>RFYVKDHRNKAMINLHIQKDNP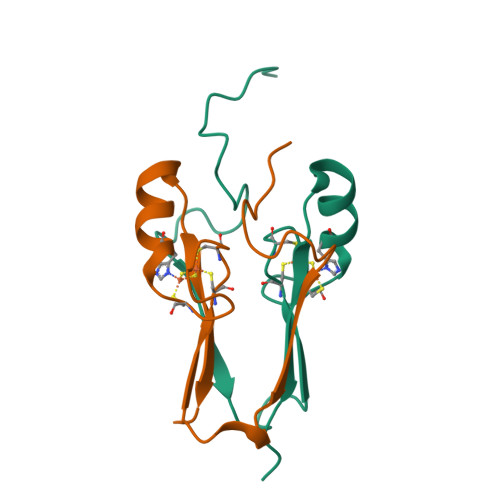KIVHAFDMEDLGDAKAVYCRCWRSKKFPFCDGAHTKHNEETGDNVGPLIIKKKET[2x]>MAHHHHHHVDDDDKMVHHDGFQTVKATIDWEHPMFKLYEKAKRNGKWNPADIDFSQDQKDFASLTSEEKISALPLVAGFSAGEEAATLDILPMAHALARQGRLEDVLFLTTFMHDEAKHVEMFSRWQQAVGIGQMDLSVFHNDHYKRIFYEALPEAMNRLYADDSPEAVIRAATVYNMIVEGTLAESGYYTFRQIYKKAGLFPGLLQGIDYLNMDEGRHIQFGIYTIQRIVNEDERYYELFIRYMDELWPHVIGYVDYLTELGKRQQQLARTYALEIDYDLLRHYVIKQFNLRKKQISRTKRVDVVEGLEKTAAES[2x]

The heterodinuclear Mn/Fe cofactor is found in the R2 subunits of subclass Ic ribonucleotide reductases (denoted as R2c) as well as a related group of proteins known as R2-like ligand-binding oxidases (R2lox). Although the physiological function of R2lox proteins is not known, the cofactor catalyzes formation of a tyrosine–valine ether cross-link in the protein scaffold. Two proteins from this group have been characterized to date, homologs from Mycobacterium tuberculosis and Geobacillus kaustophilus. Both contain the ether cross-link, and both co-purify from heterologous expression hosts with a long-chain fatty acid ligand bound in a hydrophobic channel leading from the protein surface to the active site, hence the name ligand-binding oxidase. The two metal ions are bound next to each other in octahedral geometry by two histidines and four glutamates, with the manganese ion occupying the N-terminal metal-binding site 1.

The cross-linking valine, which is completely conserved across the R2lox group, was changed to an alanine, isoleucine or leucine (V72A/I/L). Crystal structures were obtained of all three R2lox point mutants in the non-activated reduced and the oxidized resting state by soaking apo-protein crystals with MnII and FeII under anoxic or aerobic conditions, respectively. The V72A/L mutations were found to have little effect on the global structures of the reduced and oxidized resting states, but an ether cross-link was not formed in the oxidized state. In the wild-type, the hydroxyl group of Y162 is hydrogen-bonded to the carbonyl oxygen of V72 prior to cross-link formation, and this hydrogen bond is maintained in V72A/L-R2lox in the oxidized state. The mutations affect the position of the fatty acid ligand in comparison to the wild-type, likely due to decreased or increased steric constraints in the respective active site. In the oxidized state, it appears that the bridging fatty acid ligand is slightly tilted towards residue 72 in V72A- and away from it in V72L-R2lox, although these slight differences are within the range of the coordinate error. Primary or secondary carbon atoms, however, cannot be oxidized by the Mn/Fe cofactor of R2lox, likely because the resulting alkyl radical would be too unstable. The V72 mutations demonstrate that the Mn/Fe cofactor is capable of oxidizing tertiary, but neither secondary nor primary carbon atoms.> INIGNKTNENVISFFDSTDAETQNHNALMKGCGEFIVNLRTLLRTFRTITDNWILQANTKTPITDLTNTTDAQGRDYMSYLSYLYRFYRGGRRYKFFNTTPLKQSQTCYIRSFLIPRNYSADEINVDGPSHITYPVINPVHEVEVPFYSQYRKIPIASTSDKGYDSSLMYFSNTATTQIVARAGNDDFTFGWMIGPPQLQGESRSVAP;> NVHNTELASSTSENSVETQEITTFHDVETPNRIDTPMAQDTSSARNMDDTHSIIQFLQRPVLIDNIEIIAGTTADANKPLSRYVLDQQNSQKYVRSWTLPSTVLRAGGKAQKLANFKYLRCDVQVKLVLNANPFVAGRMYLAYSPYDDKVDTARSVLQTSRAGVTGYPGVELDFQLDNSVEMTIPYASFQEAYDLVTGTEDFVQLYLFPITPVLGPKSESESSKVDISVYMWLSNISLVIPTYRINP;> SKPRNQQQVCPLQNVPAWGYSLYKGIDMSVPLAYDPNNELGDLKDVFPSAVDEMAIGYVCGNPAVKHVLTWKTTDAIQKPIANGDDWGGVIPVGMPCYSKSIRTTRISATENRETEVMDAAPCEYVANMFSYWRATMCYRITVVKTAFHTGRLEIFFEPGVIPVKPTVNNIGPDQDRLTGAVAPSDNNYKYILDLTNDTEVTIRVPFVSNKMFLKTAGIYGANSENNWNFHESFSGFLCIR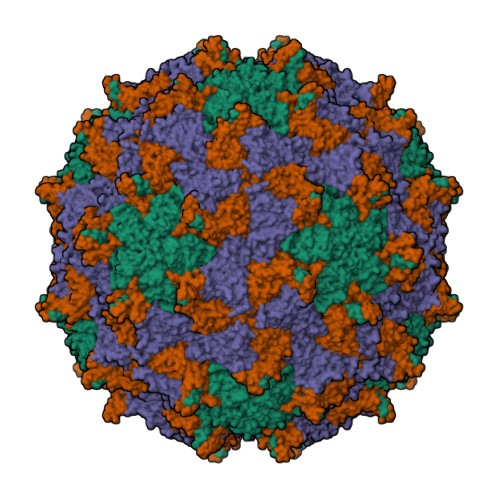PVTKLMAPDTVSDNVSIVVWKWAEDVVVVEPKPLTSGPTQVYRPPPTASTAVEVLNVEL;> TSENPKIGPISEVASGVKTTANGIERIPVIGEIAKPVTTAVKWFADVVGTVAAIFGW23-[4-(2,4,4-trimethylpentan-2-yl)phenoxy]-3,6,9,12,15,18,21-heptaoxatricosan-1-ol | C30 H54 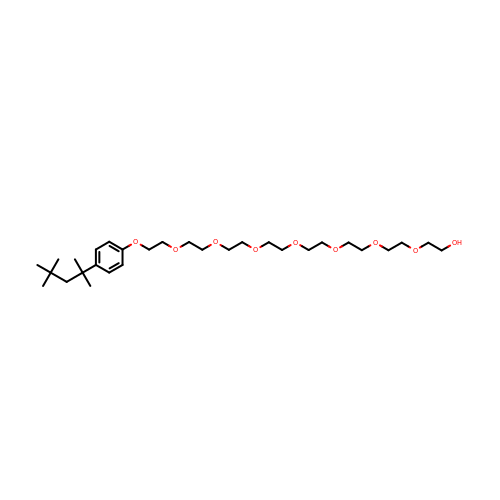O9 | OJLRAIOADFIRJN-UHFFFAOYSA-N>MAHHHHHHMKKKRVLTGDRPTGKLHLGHWIGSIMNRLQLQNDSRYDCFFIIADLHTLTTKTRKEEILQIDNHIYDVLADWLSVGIDPEKSAIYLQSAIPEIYELNLIFSMLTPLNHIMGIPSIKEMARNASLNEESLSHGLIGYPVLQSADILLAKAHLVPVGKDNEAHVELTRDIAKTFNRLYGEVFPEPDILQGELTALVGTNGQGKMSKSANNAIYLSDDAKTVQEKIRKLYTDPNRIHATTPGRVEGNPLFIYHDLFNPHK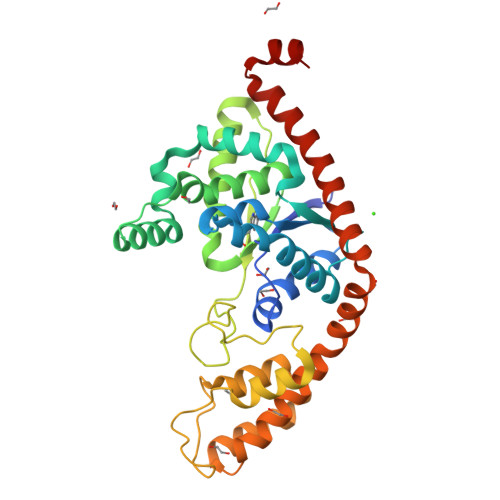EEVEEFKTRYRQGCIRDVEVKARLAEEINLFLNPFREKRSELVAQPKFLEEALQQGTEKMRTVARETMEEVHDHLGLSRKWRTILASSK[2x]>[2x]GTTGLRPSGTVSCPICMDGYSEIVQNGRLIVST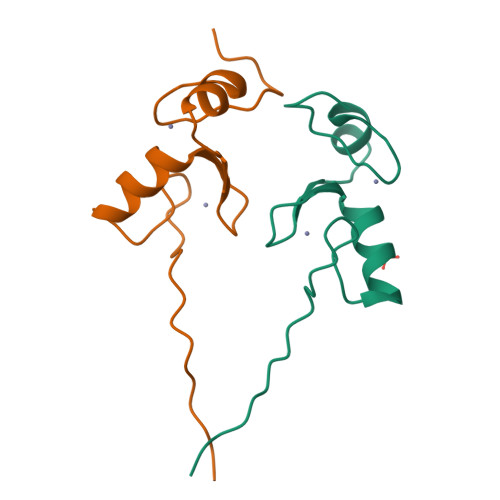ECGHVFCSQCLRDSLKNANTCPTCRKKINHKRYHPIYI>[4x]SYKVGIWGFGAMGSGIAKNILSKKNLKLVGVHDFREEYIEKDVGELLGLGKIGIKVYPDPITMVKQTDPDLVVIATNSFISVVKDQIISILKENKNVITIAEEMAFPFSKDPKAANEIDTVAKDHNVSVLGTGVNPGFVLDTLIITLTGICLNVQRIKAARINDLSPFGPTVMETQGVGTTPEEFKQGI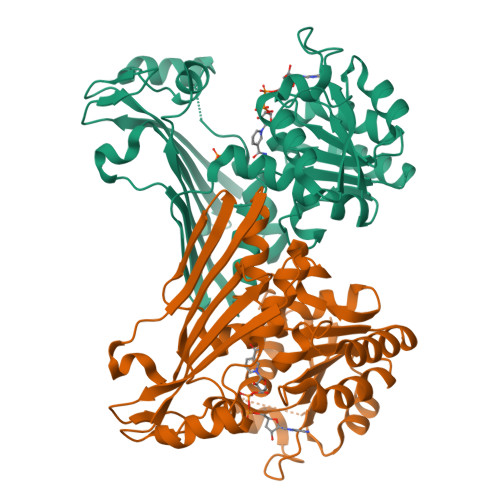KSGKIVGHIGFEQSIHMIAKALGWEIDRIEQKREPIISNVMRETKYVKVQPGMVAGCNHTAKAFYKNELLIELEHPQQVLPHLENVQTGDYITIQGDPDISMGINPEIPGGKGTIAIATNMIPSVVEARPGLLTMVDLPIPRALLAEVH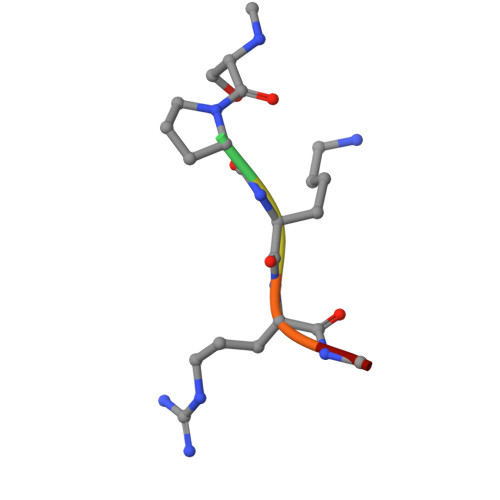> XPKRIA> MAHHHHHHMEKTLSNAAIATESISNQALPSHYNYPNSLTLKNKYGITNHKDFTNKCAHDSAKAAINLRQEEPPKKFDSSYLKYLHKQLFKETFEWAGHTRDLPFTFADGTVGVMPEMIRSNWRTEQPIIFATGNKVQDGLKNIDKMLIEKNNLQGLSHKEFIENIAEIFACLNYTHPFREGNGRTQRIFCEKLAQAAGYYLDFSV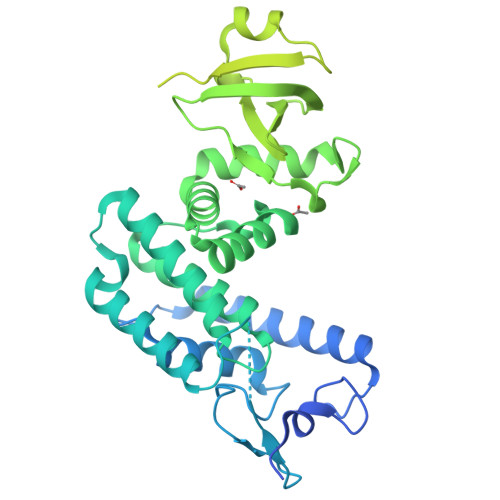VTKERMSEASITAAQDSNLEPMKKLFDDISNPIKTAVLKECINSLKNIDHKNINDCIIVAADKGLTYKGIYTDNSPDSIILKTDNIYIICSKNDLAPEQLKTLKLGDECTITVPMKQNIENTLIPKEKLPPLTKNAIIENIKKDTLIQAKLRQVTHLSKLVYGSSKILNNQLELINTNQKSGEQLSAQITSSPQSISKLAGIKIFGMKNSMRKKAEDNIIKLANSIKSYGSAVKNVETTMIQQHKSEQKRLSKTVKLPSTKLQNILNLPEEKQKEVLLEEKSLASSIGKELTDFISSLNARLSPSERKMILESNHQQFAKNVGISESQAETIIKTAQKAKEVYQKMQKPAVDLTKHLIVSG Here, we identify a novel transcription factor, CapW, that is associated with hundreds of distinct CBASS systems. We show that CapW is a transcriptional repressor that binds the promoter region of its cognate CBASS operon to inhibit expression of CBASS genes. Two structures of CapW from different bacteria reveal a dimeric assembly that likely binds a small-molecule ligand to control DNA binding and transcriptional repression. Our two structures suggest that ligand binding to the protein's WYL domain causes a conformational change in the WYL and WCX domains that triggers a large-scale rotation of the wHTH domains to release the protein from DNA.

We crystallized and determined a 2.3 Å resolution crystal structure of Pa CapW in a low-pH condition (pH 5.0). The structure reveals that Pa CapW shares the same overall architecture as Sm CapW, forming a homodimer of protomers with wHTH, WYL, and WCX domains. The symmetric arrangement of WYL domains linked by WCX domains is similar to Sm CapW, but in Pa CapW the WYL domains are each rotated ∼10° downward and inward toward the wHTH domains. This motion is accompanied by a slight widening of the groove between the WYL domains’ ligand-binding sites and bordered by the two WCX domains, and also by a rearrangement of the C-termini of each WCX domain. In Pa CapW, this region undergoes a domain swap to fold against the opposite protomer's WCX domain. Finally, we observe that a salt bridge between a conserved arginine in the WYL domain and an aspartate on the WCX domain is broken in the Pa CapW structure, enabling the WCX domain to move out and away from the dimer-related WYL domain. In our structure of Pa CapW, the WYL domains pinch inward by ∼6 Å, positioning the equivalent tryptophan residues (Trp181) and the nearby α5 helices too close to one another to accommodate the α4 helices in their original configuration. As a result, the α4 helix of each CapW protomer rotates downward away from the WYL domains. This change, and the motion of the WYL domains in general, in turn cause a striking ∼70° rotation of each wHTH domain compared to its position in Sm CapW. Whereas the wHTH domains are aligned for cooperative DNA binding in our structure of Sm CapW, in Pa CapW they are completely misaligned and would be unable to bind a contiguous DNA sequence.

> MTDESKPTDDQPTSKGRQGARWGQERRLEFIDYRLRWDGQINRSSLTDFFGISVPQASLDITEYAKLAESNLEYDTRARVYRATESFKAVFPSSAVERYLDDLLRVAVQPEIPYGSFLGWQSPVAAVPKLGRRLNADIVGVILRAIRETGFIEVFYQSLTDPEGGERMLSPHALVHDGNRWHVRAYCHKRKAFRDFSLTRIKCCKYVGQDRDRADEDYAWNTMVNVVLTPHPGLTPAQRKLIENDFLMEGGEMHVECRRALLLYLLFQLNLNEDQADQRPEVIQLALKNRDEIKDLIQY>[2x]MLPGTFFEVLKNEGVVAIATQGEDGPHLVNTWNSYLKVLDGNRIVVPVGGM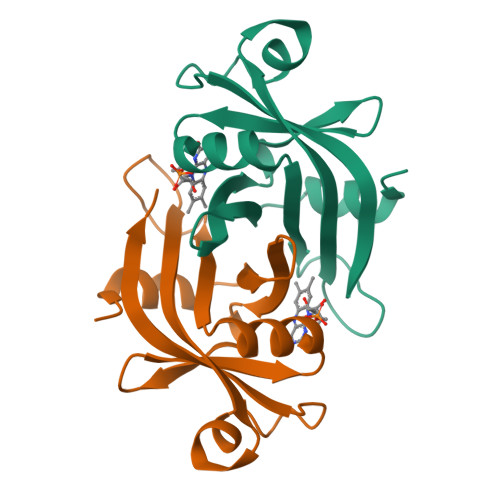HKTEANVARDERVLMTLGSRKVAGRNGPGTGFLIRGSAAFRTDGPEFEAIARFKWARAALVITVVSAEQTY> MASTANMISQLKKLSIAEPAVAKDSHPDVNIVDLMRNYISQELSKISGVDSSLIFPALEWTNTMERGDLLI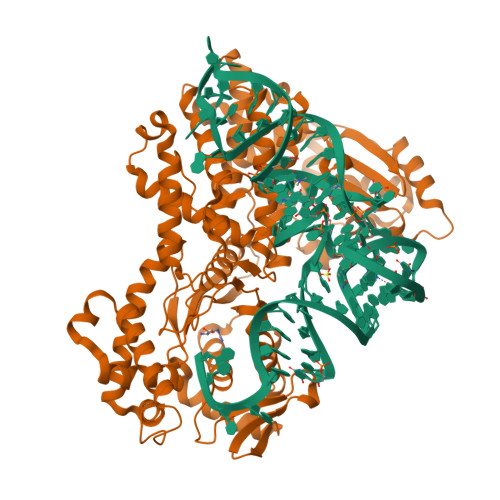PIPRLRIKGANPKDLAVQWAEKFPCGDFLEKVEANGPFIQFFFNPQFLAKLVIPDILTRKEDYGSCKLVENKKVIIEFSSPNIAKPFHAGHLRSTIIGGFLANLYEKLGWEVIRMNYLGDWGKQFGLLAVGFERYGNEEALVKDPIHHLFDVYVRINKDIEEEGDSIPLEQSTNGKAREYFKRMEDGDEEALKIWKRFREFSIEKYIDTYARLNIKYDVYSGESQVSKESMLKAIDLFKEKGLTHEDKGAVLIDLTKFNKKLGKAIVQKSDGTTLYLTRDVGAAMDRYEKYHFDKMIYVIASQQDLHAAQFFEILKQMGFEWAKDLQHVNFGMVQGMSTRKGTVVFLDNILEETKEKMHEVMKKNENKYAQIEHPEEVADLVGISAVMIQDMQGKRINNYEFKWERMLSFEGDTGPYLQYAHSRLRSVERNASGITQEKWINADFSLLKEPAAKLLIRLLGQYPDVLRNAIKTHEPTTVVTYLFKLTHQVSSCYDVLWVAGQTEELATARLALYGAARQVLYNGMRLLGLTPVERM>MSLIPKFRAWDTYEKEMLENVTPLFDDSNSMIAIITDFQIKGSPGTSEIEIGSYDTTFNWDEFPYVIMQSTGLKDKNGVEIFEGDILVYDAPKKYAHRRSMHEIAYADGRFFWEFLD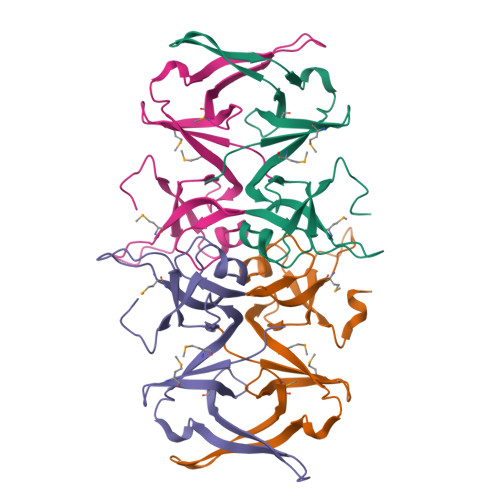LVFCQSNILYRDGYLVIGNIHENPELLEGNEGHHHHHH[4x]> MPFVNKQFNYKDPVNGVDIAYIKIPNAGQMQPVKAFKIHNKIWVIPERDTFTNPEEGDLNPPPEAKQVPVSYYDSTYLSTDNEKDNYLKGVTKLFERIYSTDLGRMLLTSIVRGIPFWGGSTIDTELKVIDTNCINVIQPDGSYRSEELNLVIIGPSADIIQF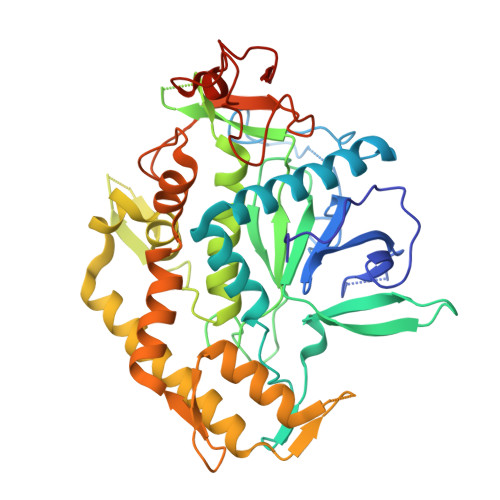ECKSFGHEVLNLTRNGYGSTQYIRFSPDFTFGFEESLEVDTNPLLGAGKFATDPAVTLAHELIHAGHRLYGIAINPNRVFKVNTNAYYEMSGLEVSFEELRTFGGHDAKFIDSLQENEFRLYYYNKFKDIASTLNKAKSIVGTTASLQYMKNVFKEKYLLSEDTSGKFSVDKLKFDKLYKMLTEIYTEDNFVKFFKVLNRKTYLNFDKAVFKINIVPKVNYTIYDGFNLRNTNLAANFNGQNTEINNMNFTKLKNFTPLVPR>MEAFEISDFKEHAKKKSMWAGALNKVTISGLMGVFTEDEDLMALPIHRDHCPALLKIFDEIIVNATDHERACHNKTKKVTYIKISFDKGVFSCENDGPGIPIAKHEQASLIAKRDVYVPEVASCHFLAGTNINKAKDCIKGGTNGVGLKLAMVHSQWAILTTADGAQKYVQHINQRLDIIEPPTITPSREMFTRIELMPVYQELGYAEPLSETEQADLSAWIYLRACQCAAYVGKGTTIYYNDKPCRTGSVMALAKMYTLLSAPNSTIHTATIKADAKPYSLHPLQVAAVVSPKFKKFEHVSVINGVNCVKGEHVTFLKKTINEMVVKKFQQTIKDKNRKTTLRDSCSNIFIVIVGSIPGIEWTGQRKDELSIAENVFKTHYSIPSSFLTSMTKSIVDILLQSISKKDNHKQVDVDKYTRARNAGGKRAQDCMLLAAEGDSALSLLRTGLTLGKSNPSGPSFDFCGMISLGGVIMNACKKVTNITTDSGETIMVRNEQLTNNKVLQGIVQVLGLDFNCHYKTQEERAKLRYGCIVACVDQDLDGCGKILGLLLAYFHLFWPQLIIHGFVKRLLTPLIRVYEKGKTMPVEFYYEQEFDAWAKKQTSLANHTVKYYKGLAAHDTHEVKSMFKHFDNMVYTFTLDDSAKELFHIYFGGESELRKRELCTGVVPLTETQTQSIHSVRRIPCSLHLQVDTKAYKLDAIERQIPNFLDGMTRARRKILAGGVKCFASNNRERKVFQFGGYVADHMFYHHGDMSLNTSIIKAAQYYPGSSHLYPVFIGIGSFGSRHLGGKDAGSPRYISVQLASEFIKTMFPAEDSWLLPYVFEDGQRAEPEYYVPVLPLAIMEYGANPSEGWKYTTWARQLEDILALVRAYVDKDNPKHELLHYAIKHKITILPLRPSNYNFKGHLKRFGQYYYSYGTYVISEQRNIITITELPLRVPTVAYIESIKKSSNRMTFIEEIIDYSSSETIEILVKLKPNSLNRIVEEFKETEEQDSIENFLRLRNCLHSHLNFVKPKGGIIEFNTYYEILYAWLPYRRELYQKRLMREHAVLKLRIIMETAIVRYINESAELNLSHYEDEKEASRILSEHGFPPLNHTLIISPEFAS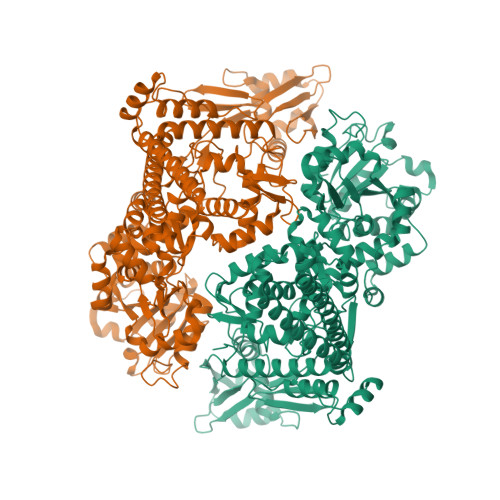IEELNQKALQGCYTYILSLQARELLIAAKTRRVEKIKKMQARLDKVEQLLQESPFPGASVWLEEIDAVEKAIIKGRNTQWKFH[2x]> MHHHHHHMFSRFSNVVSEIEKKYVDKISISEIMTKAIEGLLSNLDAHSAYLNEKKFKEFQAQTEGEFGGLGITVGMRDGVLTVIAPLEGTPAYKAGVKSGDNILKINNESTLSMSIDDAINLMRGKPKTPIQI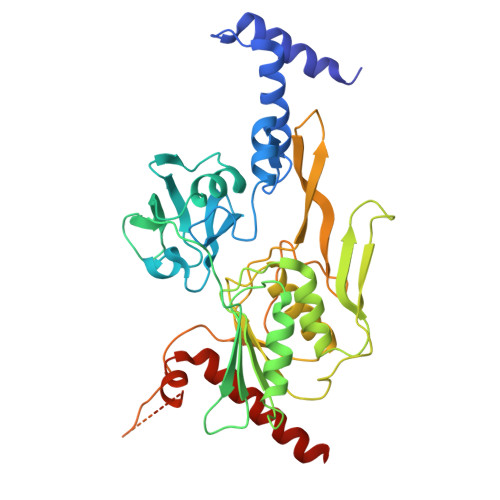TIVRKNEPKPLVFNIIRDIIKLPSVYVKKIKETPYLYVRVSGFDKNVTKSVLEGLKANPKAKGIVLDLRGNPGGLLNQAVGLSNLFIKEGVLVSQKGKNKEESLEYKANGRAPYTNLPIAVLVNGGSASASEIVAGALQDHKRAVIIGEKTFGKGSVQMLLPVNKDEAIKITTARYYLPSGRTIQAKGITPDIVIYPGKVPENENKFSLKEADLKHHLEQELKKLDDKTPNSKEADKDKKNEEEKEVTPKMINDDIQLKTAIDSLKTWSIVDEKMDEKAPKKK Stl, the master repressor of the Staphylococcus aureus pathogenicity islands (SaPIs), targets phage-encoded proteins to derepress and synchronize the SaPI and the helper phage life cycles. Our previous work has shown that the Stl repressor, an all-alpha helix protein, is a modular protein composed of an N-terminal domain with the characteristic helix-turn-helix (HTH) folding, which mediates DNA binding, followed by a middle and a C-terminal dimerization domain. Trimeric Duts show high sequence conservation at the residues that make up their active centers, which has been used to define five catalytic motifs (motifs I to V) that are the signature of this family of enzymes. For all these Dut-StlN-ter complexes, the Dut maintains its trimeric state and binds three independent Stl monomers, each of which uses predominantly its middle domain to interact with individual active centers of trimeric Dut.

The mDut-StlN-ter complex was crystallized in the space group P21, and the crystal asymmetric unit contains two mDut trimers and six StlN-ter monomers, forming two mDut-StlN-ter complexes with a 1:1 stoichiometry in which each mDut trimer interacts with three independent StlN-ter protomers. In the mDut-StlN-ter structure, the two independent complexes are largely identical with a root mean square deviation (RMSD) of 1.1 Å for the superimposition of 642 Cα atoms corresponding to the Dut trimer and the three StlN-ter protomers. In both complexes, clear and traceable electron density is present for the entire Dut protomers, except for the eight C-terminal residues corresponding to the catalytic P-loop motif V, which covers the active center of the enzyme once the nucleotide has been bound. In the complex, the Dut active center is occupied by the StlN-ter molecule, forcing the projection of this P-loop into the solvent. Interestingly, a detailed view of this structural comparison shows that the trimer of mDut in complex with Stl is more similar to the nucleotide-bound form than the apo form. The differences are mainly concentrated in the unique and short α helix (mDut residues 65 to 70) from the catalytic motif III. In the Apo mDut, this helix is distorted, losing its helical topology, whereas in the nucleotide- and Stl-bound forms it folds as identical α helices. This observation indicates that Stl recognizes the Dut active center in its competent conformation for nucleotide binding, in agreement with the capacity of Stl to inhibit the enzymatic activity of Dut. In contrast, the absence of motif VI is exploited in the complex with mDut where Y116 presents, in the different Stl subunits, rotameric conformations alternative to that observed in the ϕ11Dut and hDut complexes. As in phage and human complexes, Y116 from some Stl protomers interacts with mDut D109 and R110, but in other protomers, the rotamer is identical to that observed in the Stl free form, losing these interactions and forming new ones with L67 and R70 in motif II.

>AELPTHYGTIIKTLRKYMKLTQSKLSERTGFSQNTISNHENGNRNIGVNEIEIYGKGLGIPSYILHRISDEFKEKGYSPTLNDFGKFDKMYSYVNKAYYNDGDIYYSSYDLYDETIKLLELLKESKINVNDIDYDYVLKLYKQILST[6x];>[6x]MSTTLAIVRLDPGLPLPSRAHDGDAGVDLYSAEDVELAPGRRALVRTGVAVAVPFGMVGLVHPRSGLATRVGLSIVNSPGTIDAGYRGEIKVALINLDPAAPIVVHRGDRIAQLLVQRVELVELVEVSSFDEAGLA>MSEEPVQSNMDISTGHMILSYMEDHLKNKNRLEKEWEALC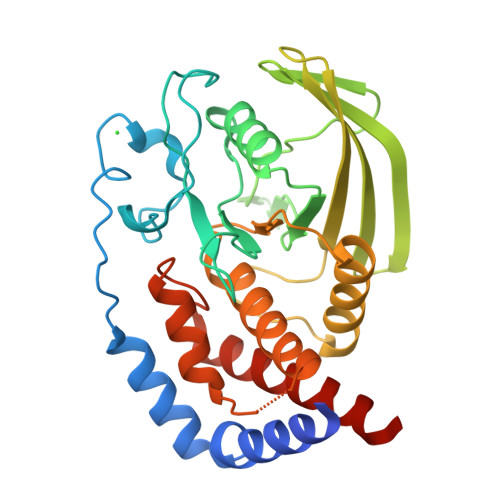AYQAEPNSSFVAQREENVPKNRSLAVLTYDHSRVLLKAENSHSHSDYINASPIMDHDPRNPAYIATQGPLPATVADFWQMVWESGCVVIVMLTPLAENGVRQCYHYWPDEGSNLYHIYEVNLVSEHIWCEDFLVRSFYLKNLQTNETRTVTQFHFLSWYDRGVPSSSRSLLDFRRKVNKCYRGRSCPIIVHCSDGAGRSGTYVLIDMVLNKMAKGAKEIDIAATLEHLRDQRPGMVQTKEQFEFALTAVAEEVNAILAHHHHHH[2x]>XG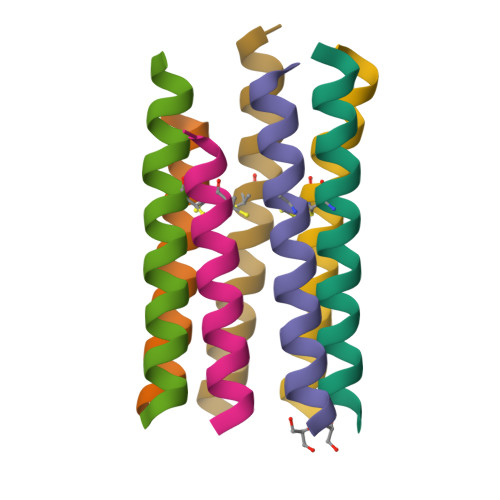EIAKALREIAKALRECAWAHREEAKALRG[7x]> GMD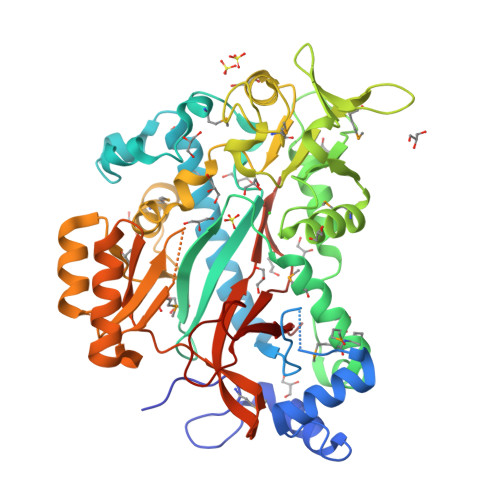TAKTKPFDEMFLQDEVIRPIYAEYAAWLQDVPHQQLESKRQEAELLFRRVGITFNVYGEDAGAERLIPFDVVPRILSASEWARLSDGAIQRVKALNMFLHDVYHDQEIIKAGIVPSSILANAQYRPEMFGVDVPGGVYAHIAGVDLVRTGENDFYVLEDNLRTPSGVSYMLENRKMMMRLFPELFRRYPVAPVEHYPQVLLNNLRAVAQAGVHEPTVVLLTPGAYNSAYFEHAFIAQQMGIELVEGQDLFVRNNAVYMRTTEGPKRVDVIYRRIDDDFIDPLSFRPDSMLGVPGLLSVYRNGGVTLANAVGTGVADDKDTYIYVPEMIRFYLGEEPILSNVPTYQLSKADDLKYVLDNLAELVVKEVQGSGGYGMLVGPAASKQELEDFRQRILANPANYIAQPTLALSTCPTLVETGIAPRHVDLRPFVLSGKTVSLVPGALCRVALREGSLVVNSSQGGGTKDTWILKD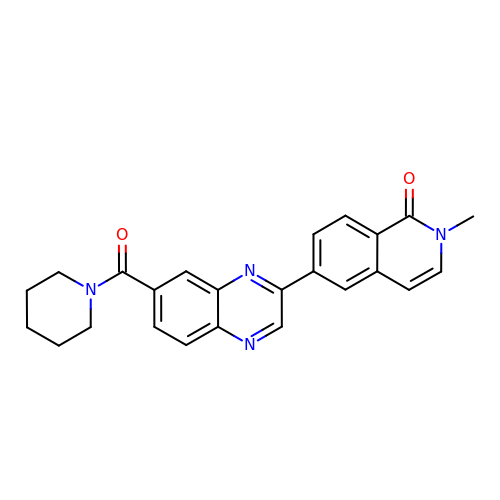2-methyl-6-[7-(piperidine-1-carbonyl)quinoxalin-2-yl]isoquinolin-1(2H)-one | C24 H22 N4 O2 | URHPFANOQLIROT-UHFFFAOYSA-N~{N}-[(1~{R})-1-(3-aminophenyl)ethyl]-6,7-dimethoxy-2-methyl-quinazolin-4-amine | C19 H22 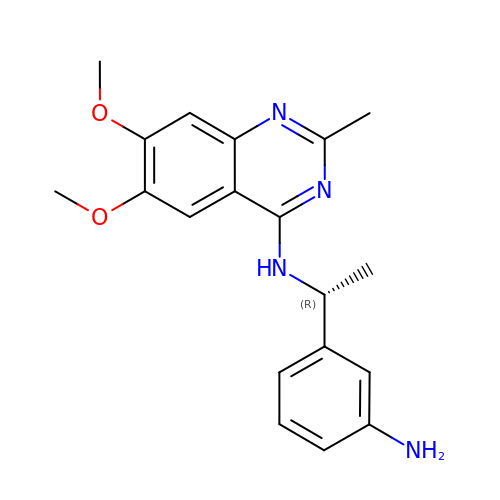N4 O2 | MNDALSIIIRYSTC-LLVKDONJSA-N> GAMGSMSKSLKKLVEESREKNQPEVDMSDRGISNMLDVNGLFTLSHITQLVLSHNKLTMVPPNIAELKNLEVLNFFNNQIEELPTQISSLQKLKHLNLGMNRLNTLPRGFGSLPALEVLDLTYNNLSENSLPGNFFYLTTLRALYLSDNDFEILPPDIGKLTKLQILSLRDNDLISLPKEIGELTQLKELHIQGNRLTVLPPELGNLDLTGQKQVFKAENNPWVTPIADQFQLGVSHVFEYIRSETYKYLYGRHMQANPEPPKKNNDKSKKISRKPLAAKNR;> GPGSMGVPICGACRRPIEGRVVNAMGKQWHVEHFVCAKCEKPFLGHRHYERKGLAYCETHYNQLFGDVCFHCNRVIEGDVVSALNKAWCVNCFACSTCNTKLTLKNKFVEFDMKPVCKKCYEKFPLELKKRLKKLAE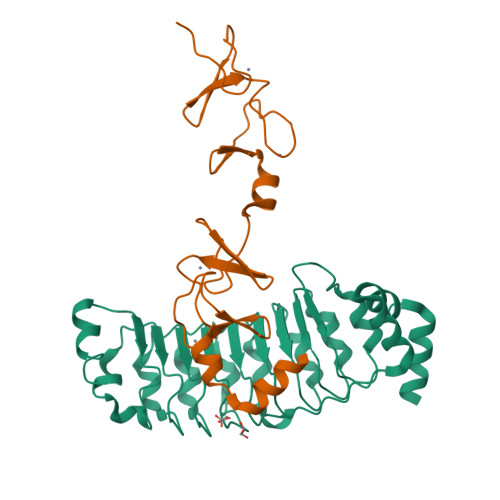TLGRK> SNAEQVRQAGIDDIGGILELIHPLEEQGILVRRSREQLEQEIGKFTIIEKDGLIIGCAALYPYSEERKAEMACVAIHPDYRDGNRGLLLLNYMKHRSKSENINQIFVLTTH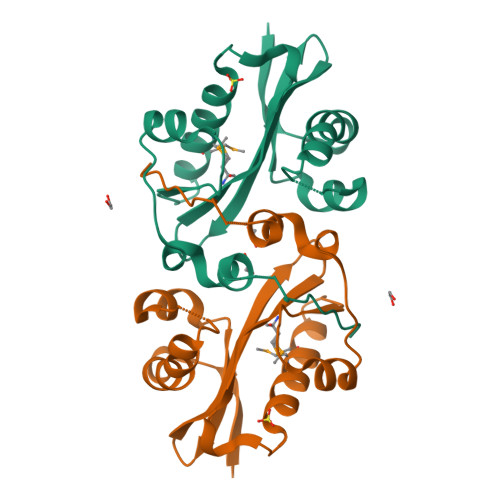SLHWFREQGFYEVGVDYLPGAKQGLYNFQRKSKILALDL N1-CYCLOPENTYL-N2-(THIAZOL-2-YL)OXALAMIDE | C10 H13 N3 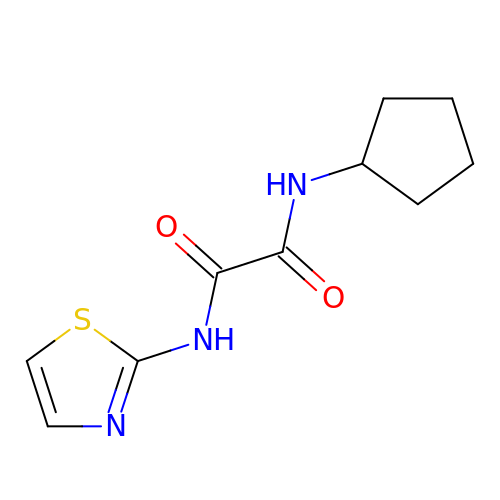O2 S | BJHPYHUDDCVBNG-UHFFFAOYSA-N Here we present a strategy for fusing small RNAs to a group II intron that yields high resolution structures of the appended RNA. Group II introns are self-splicing catalytic RNAs that have six distinct domains and typically range in size from 400 to 850 nucleotides. Our versatile scaffolding strategy enables efficient RNA structure determination for a broad range of small to moderate-sized RNAs, which were previously intractable for high-resolution cryo-EM studies.

We then tested the ability of the group IIC intron in isolation to function as a scaffold. The O.i. intron folds into a stable structure that crystallizes in a wide variety of precipitants. However, this particular intron has the unwanted tendency to undergo intramolecular hydrolytic cleavage at multiple sites, which may also cleave an attached RNA target. We therefore used an inactive mutant in which an active site residue is mutated to abolish catalytic activity. In our first attempt, we obtained a reconstruction at 2.4 Å resolution for this group II intron. In addition, this intron exhibited a very favorable lack of orientation preference and has a stable solvent-exposed stem that could be used to embed an RNA of interest (domain III). The orientation distribution map is evenly populated, which is highly unusual for a protein-free RNA in our experience. Domain III (gold) forms a stable stem loop that extends away from the rest of the folded RNA. C A local resolution map shows that the core of the scaffold has a resolution of 2.4 Å. The plot is evenly populated indicating that the group IIC intron scaffold exhibits no preferred orientation.

> GUUAUGUGUGCCCGGCAUGGGUGCAGUCUAUAGGGUGAGAGUCCCGAACUGUGAAGGCAGAAGUAACAGUUAGCCUAACGCAAGGGUGUCCGUGGCGACAUGGAAUCUGAAGGAAGCGGACGGCAAACCUUCGGUCUGAGGAACACGAACUUCAUAUGAGGCUAGGUAUCAAUGGAUGAGUUUGCAUAACAAAACAAAGUCCUUUCUGCCAAAGUUGGUACAGAGUAAAUGAAGCAGAUUGAUGAAGGGAAAGACUGCAUUCUUACCCGGGGAGGUCUGGAAACAGAAGUCAGCAGAAGUCAUAGUACCCUGUUCGCAGGGGAAGGACGGAACAAGUAUGGCGUUCGCGCCUAAGCUUGAACCACCGUAUACCGAACGGUACGUACGGUGGUGUGAGAGGAGUUCGCUCUACUCUAU>GHMA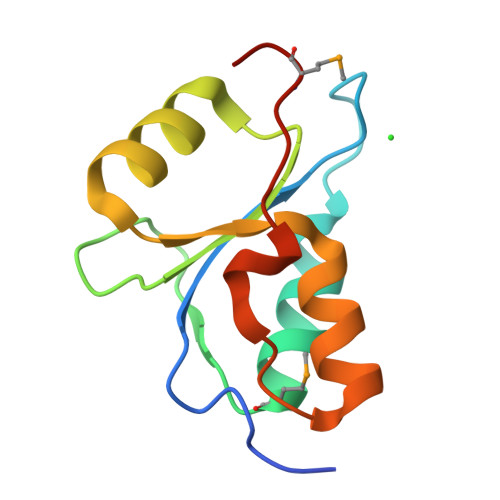APILKDVVAYVEVWSSNGTENYSKTFTTQLVDMGAKVSKTFNKQVTHVIFKDGYQSTWDKAQKRGVKLVSVLWVEKCRTAGAHIDESLFPAANMNEHLS[3x]> UUGCCAUGUGUAUGUGGG;> CCCACAUACUUUGUU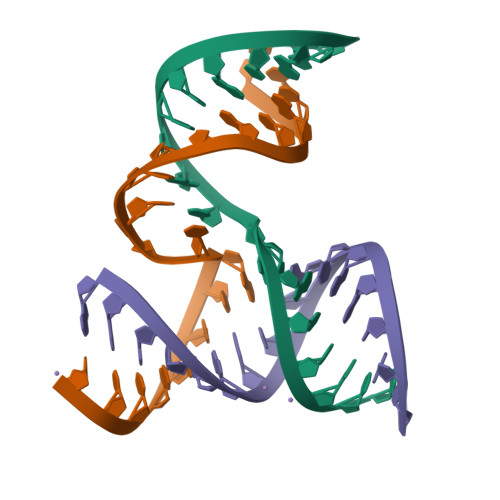GAUCC;> GGAUCAAUCAUGGCAA>[2x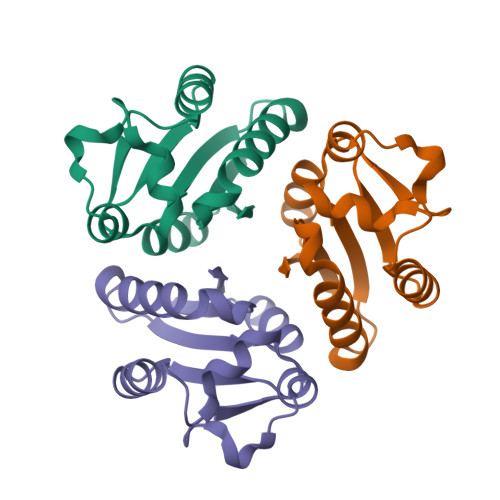]MKVVVQIKDFDKVPQALRSVINLYNDIKDAEIEVVLHQSAIKALLKDSDTRSIIEDLIKKNILIVGCENSIRSQNLSHDQLIPGIKIVTSGVGEIVRKQSEGWIYLAL PB1 domains are protein interaction modules with critical roles in the assembly of protein complexes involved in autophagy, signaling, cell division, and redox processes, as well as the auxin-response pathway in plants. PB1 domains form homotypic interactions via conserved electrostatic motifs molded by basic or acidic surface patches on opposite faces of their ubiquitin-like β-grasp fold. While type A and type B PB1 domains can form heterodimeric protein complexes, type AB members can mediate interactions with either PB1 domain type or engage in homotypic interactions to form homo-oligomers or hetero-oligomers. Our cryo-EM structures of filamentous p62 and AtNBR1–PB1 assemblies revealed that the presence of a tandem arginine sequence in the basic motif of type AB interfaces is required to stabilize a polymeric assembly.

Of the three PB1 assemblies studied, AtNBR11–94 (AtNBR1–PB1) and p621–122 (p62-PB1) formed homogeneous filaments of constant diameter that appeared best suited for high-resolution structure investigation by cryo-EM. Image classification of segmented PB1 helices revealed that both AtNBR1–PB1 and p62-PB1 polymerize in two different tubular morphologies: a projection class with a ladder-like pattern, we term L-type, and a projection class with a serpent-like one, we term S-type. For p62-PB1, we observed a four-stranded L-type assembly and a three-stranded S-type assembly. The L-type here has a pitch of 135.9 Å with 14.16 subunits/turn, and S-type has a pitch of 138.6 Å with 13.60 subunits/turn. Using the derived symmetries, we determined the 3.5/3.9- (L-type, p62/AtNBR1) and 4.0/4.4 Å- (S-type, p62/AtNBR1) resolution structures. All four structures form tubules of ~120 Å and 150-Å width with an inner diameter of 45 Å and 70 Å for AtNBR1–PB1 and p62-PB1, respectively. The overall fold of the asymmetric unit was found compatible with the NMR structure of the p62-PB1 monomer. The β1–α1 loop in p62 is flexible and only visible in the L-type assembly density. The main interactions are formed between a double arginine finger formed by two neighboring arginine residues in strand β2 (R19–R20AtNBR1/R21–22p62) stabilizing strong salt bridges to acidic residues (D60/D62/D64/D73AtNBR1 or D69/D71/D73/E82p62) in the OPCA motif located in the β2–β3 loop and the α2 helix. In addition to the canonical transverse interactions, the helices are further stabilized by longitudinal interactions Y14AtNBR1/N28AtNBR1 or K102p62/D92p62 and R59p62/D93p62 to subunits of neighboring strands along the helical axis.

> MASLTVKAYLLGKEDAAREIRRFSFCCSPEPEAEAEAAAGPGPCERLLSRVAALFPALRPGGFQAHYRDEDGDLVAFSSDEELTMAMSYVKDDIFRIYIKEKKECRRDHRPPCAQEAPRNMV>[2x]GPH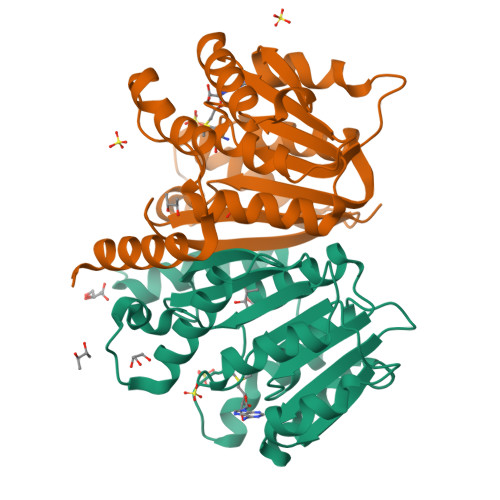MMEQERWNSVDVYFSSLLVKEDEALSKAAQAHREFDLPDLAVSAPQGKLLHLLARLRQARRILEIGTFGGYSSIWLARALPPDGRLVTIEWERSFAESAASRLAEAGVAHLVEQHVGRALDILPTLDRPGTAPFDMVFVDANKPDIPEYFTWALKLSRPGAVVVVDNVVLGGAVTDPDHPDAGVQGVRRFHEMLAGRSDVTATSIQTVGTKGYDGFTLALVTG(2-{[(2S)-1-hydroxy-3-(6-oxo-1,6-dihydro-9H-purin-9-yl)propan-2-yl]oxy}ethyl)phosphonic 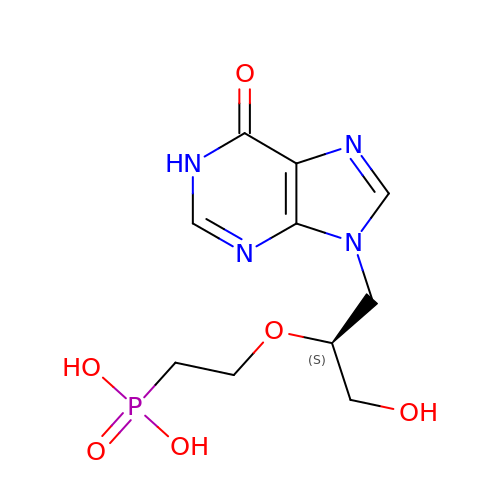acid | C10 H15 N4 O6 P | KECBSFFYQIGYIU-ZETCQYMHSA-N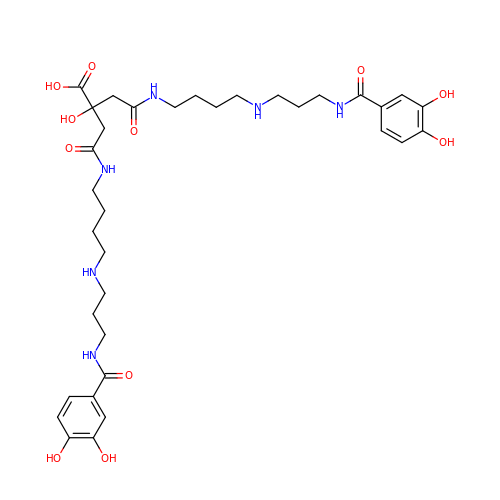4-[4-[3-[[3,4-bis(oxidanyl)phenyl]carbonylamino]propylamino]butylamino]-2-[2-[4-[3-[[3,4-bis(oxidanyl)phenyl]carbonylamino]propylamino]butylamino]-2-oxidanylidene-ethyl]-2-oxidanyl-4-oxidanylidene-butanoic acid | C34 H50 N6 O11 | GKIMOVAPSAVJHZ-UHFFFAOYSA-N>SMSLQVNLLNNTFANPFMNAAGVMCTTTEELVAMTESASGSLVSKSCTPALREGNPTPRYQALPLGSINSMGLPNNGFDFYLAYAAEQHDYGKKPLFLSMSGLSMRENVEMCKRLAAVAT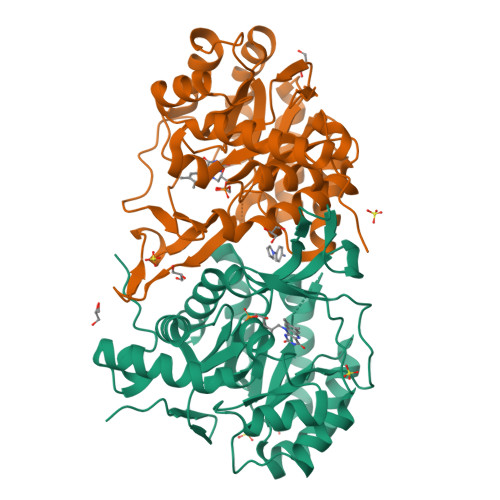EKGVILELNLSCPNVPGKPQVAYDFDAMRQCLTAVSEVYPHSFGVKMPPYFDFAHFDAAAEILNEFPKVQFITCINSIGNGLVIDAETESVVIKPKQGFGGLGGRYVLPTALANINAFYRRCPGKLIFGCGGVYTGEDAFLHVLAGASMVQVGTALQEEGPSIFERLTSELLGVMAKKRYQTLDEFRGKVRTLDGTAESTR[2x]> GAMGYKDNIRHGVCWIYYPDGGSLVGEVNEDGEMTGEKIAYVYPDERTALYGKFIDGEMIEGKLATLMSTEEGRPHFELMPGNSVYHFDKSTSSCISTNALLPDPYESERVYVAESLISSAGEGLFSKVAVGPNTVMSFYNGVRITH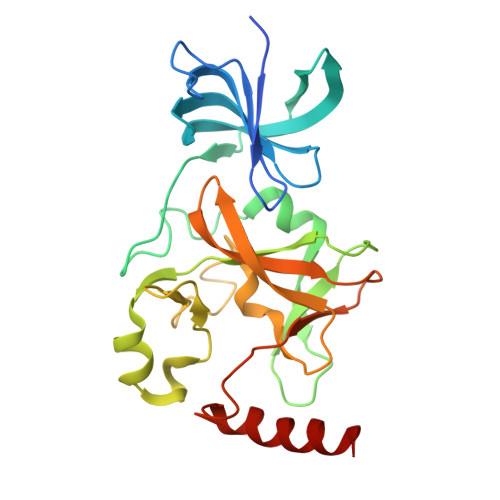QEVDSRDWALNGNTLSLDEETVIDVPEPYNHVSKYCASLGHKANHSFTPNCIFDMFVHPRFGPIKCIRTLRAVEADEELTVAYGYDHSPPGKSGPEAPEWYQVELKAFQATQQK>GPMTDISMGDLHANALLFLNILVRQGIIAISPENYAKFAEIYTLPELQADYWGTEAPVFSAENKQERLEEIKKQYNALIAQIKIINTKKLIRLIGDELVDRGVIDYFILKLLQALYDQGADFEILLSNHGIEFVEACELFKENGNKLVAKRLGNIQHGNSFHALQEAIAAGAISNEEVLNIYHQVYKKHLKIISYSLDPDANEIKVFSHAGIGLNHIRGLARKFKVPYSEESAVDLAKTIDAINKKFAEKASSGEIHTLYTHDMMYRGYAGEHLNSTDEVVAATVWGREYGDLIRTSKKFKITFIHGHDSYDPEKVEHVTLN[2x]

IcmW-Interacting Protein B (WipB) is a 60 kDa Legionella effector of unknown function originally identified amongst a cohort of proteins that interact with the Dot/Icm T4S chaperone complex IcmS/IcmW10. Our data reveal that WipB is a modular effector, with an N-terminal Ser/Thr phosphatase domain related to the eukaryotic phospho-protein phosphatase (PPP) family, and a C-terminal domain sufficient to pilot WipB to the acidified LAMP1-positive lysosomal compartments in eukaryotic cells, where WipB interacts with the v-ATPase and the associated LAMTOR1 phosphoprotein, key components of the lysosomal nutrient sensing (LYNUS) apparatus. We propose that WipB is a lysosome-targeted phosphatase that modulates cellular nutrient sensing and the control of energy metabolism during Legionella infection.

The crystal structure of the N-terminal domain at 1.7 Å resolution comprising residues 25 to 344 revealed that WipB harbours a Ser/Thr phosphatase domain related to the eukaryotic phospho-protein phosphatase (PPP) family. The resulting fragment, WipB25-344, also yielded a stable protein, which in contrast to WipB1-364 crystallised readily. The structure was solved using the Molecular Replacement method, with the recently solved structure of WipA (a protein with 34% identity at amino acid sequence level) serving as a search model. WipB25-344 crystallizes as a dimer in the asymmetric unit. In chain A, density for residues 332–344 is missing while the same region is resolved in chain B, This region in chain B interacts with chain A, probably an artefact of crystal packing as WipB25-344 is monomeric in solution. The structure of WipB25-344 is very similar to that of WipA24-435 determined previously (the structures align with a root-mean-square deviation in Cα atoms of 1.9 Å over 279 WipB residues). In the PPP family, the DxH, GDxxDR, and NHE signature motifs are strictly conserved and comprise most of the residues that form the catalytic site14 WipB exhibits similar motifs, namely GDLHA, GDELVDR, and NHG, and these motifs cluster in one particular region of WipB25-244, on the loops connecting β1 and α1 (GDLHA), β2 and α4 (GDELVDR), and β3 and α5 (SNG). In WipB, Arg310 (equivalent of Arg369 in WipA), is conformationally restrained away from the active site and therefore cannot assume a role in substrate recognition.> MAQQTPLYEQHTLCGARMVDFHGWMMPLHYGSQIDEHHAVRTD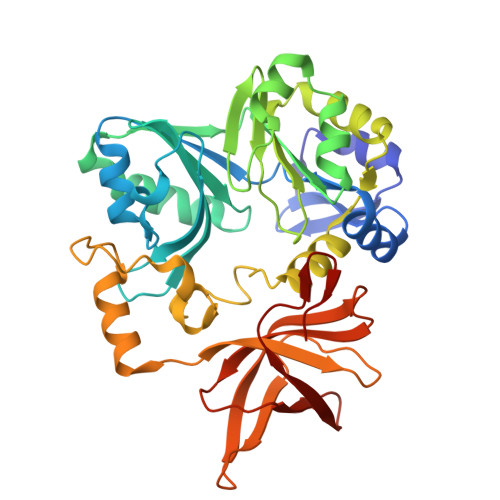AGMFDVSHMTIVDLRGSRTREFLRYLLANDVAKLTKSGKALYSGMLNASGGVIDNLIVYYFTEDFFRLVVNSATREKDLSWITQHAEPFGIEITVRDDLSMIAVQGPNAQAKAATLFNDAQRQAVEGMKPFFGVQAGDLFIATTGYTGEAGYEIALPNEKAADFWRALVEAGVKPCGLGARDTLRLEAGMNLYGQEMDETISPLAANMGWTIAWEPADRDFIGREALEVQREHGTEKLVGLVMTEKGVLRNELPVRFTDAQGNQHEGIITSGTFSPTLGYSIALARVPEGIGETAIVQIRNREMPVKVTKPVFVRNGKAVA>MAQSMYPNEPIVVVGSGCRFPGDANTPSKLWELLQHPRDVQSRIPKERFDVDTFYHPDGKHHGRTNAPYAYVLQDDLGAFDAAFFNIQAGEAESMDPQHRLLLETVYEAVTNAGMRIQDLQGTSTAVYVGVMTHDYETVSTRDLESIPTYSATGVAVSVASNRISYFFDWHGPSMTIDTACSSSLVAVHLAVQQLRTGQSSMAIAAGANLILGPMTFVLESKLSMLSPSGRSRMWDAGADGYARGEAVCSVVLKTLSQALRDGDTIECVIRETGVNQDGRTTGITMPNHSAQEALIKATYAQAGLDITKAEDRCQFFEAHGTGTPAGDPQEAEAIATAFFGHEQVARSDGNERAPLFVGSAKTVVGHTEGTAGLAGLMKASFAVRHGVIPPNLLFDKISPRVAPFYKNLRIPTEATQWPALPPGQPRRASVNSFGFGGTNAHAIIEEYMEPEQNQLRVSNNEDCPPMTGVLSLPLVLSAKSQRSLKIMMEEMLQFLQSHPEIHLHDLTWSLLRKRSVLPFRRAIVGHSHETIRRALEDAIEDGIVSSDFTTEVRGQPSVLGIFTGQGAQWPGMLKNLIEASPYVRNIVRELDDSLQSLPEKYRPSWTLLDQ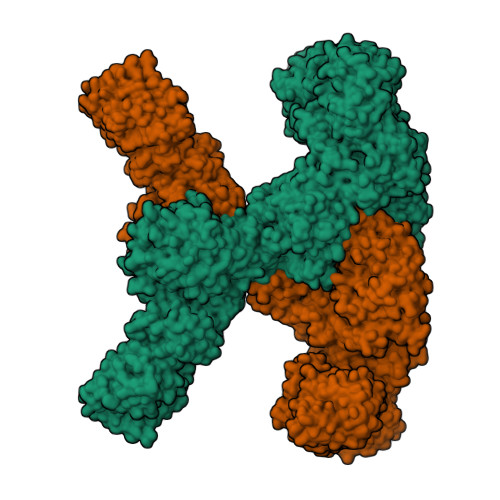FMLEGEASNVQYATFSQPLCCAVQIVLVRLLEAARIRFTAVVGHSSGEIACAFAAGLISASLAIRIAYLRGVVSAGGARGTPGAMLAAGMSFEEAQEICELDAFEGRICVAASNSPDSVTFSGDANAIDHLKGMLEDESTFARLLKVDTAYHSHHMLPCADPYMQALEECGCAVADAGSPAGSVPWYSSVDAENRQMAARDVTAKYWKDNLVSPVLFSHAVQRAVVTHKALDIGIEVGCHPALKSPCVATIKDVLSGVDLAYTGCLERGKNDLDSFSRALAYLWERFGASSFDADEFMRAVAPDRPCMSVSKLLPAYPWDRSRRYWVESRATRHHLRGPKPHLLLGKLSEYSTPLSFQWLNFVRPRDIEWLDGHALQGQTVFPAAGYIVMAMEAALMIAGTHAKQVKLLEILDMSIDKAVIFDDEDSLVELNLTADVSRNAGEAGSMTISFKIDSCLSKEGNLSLSAKGQLALTIEDVNPRTTSASDQHHLPPPEEEHPHMNRVNINAFYHELGLMGYNYSKDFRRLHNMQRADLRASGTLDFIPLMDEGNGCPLLLHPASLDVAFQTVIGAYSSPGDRRLRCLYVPTHVDRITLVPSLCLATAESGCEKVAFNTINTYDKGDYLSGDIVVFDAEQTTLFQVENITFKPFSPPDASTDHAMFARWSWGPLTPDSLLDNPEYWATAQDKEAIPIIERIVYFYIRSFLSQLTLEERQQAAFHLQKQIEWLEQVLASAKEGRHLWYDPGWENDTEAQIEHLCTANSYHPHVRLVQRVGQHLLPTVRSNGNPFDLLDHDGLLTEFYTNTLSFGPALHYARELVAQIAHRYQSMDILEIGAGTGGATKYVLATPQLGFNSYTYTDISTGFFEQAREQFAPFEDRMVFEPLDIRRSPAEQGFEPHAYDLIIASNVLHATPDLEKTMAHARSLLKPGGQMVILEITHKEHTRLGFIFGLFADWWAGVDDGRCTEPFVSFDRWDAILKRVGFSGVDSRTTDRDANLFPTSVFSTHAIDATVEYLDAPLASSGTVKDSYPPLVVVGGQTPQSQRLLNDIKAIMPPRPLQTYKRLVDLLDAEELPMKSTFVMLTELDEELFAGLTEETFEATKLLLTYASNTVWLTENAWVQHPHQASTIGMLRSIRREHPDLGVHVLDVDAVETFDATFLVEQVLRLEEHTDELASSTTWTQEPEVSWCKGRPWIPRLKRDLARNNRMNSSRRPIYEMIDSSRAPVALQTARDSSSYFLESAETWFVPESVQQMETKTIYVHFSCPHALRVQALGFFYLVQGHVQEGNREVPVVALAERNASIVHVRPDYIYTEADNNLSEGGGSLMVTVLAAAVLAETVISTAKCLGVTDSILVLNPPSICGQMLLHAGEEIGLQVHLATTSGNRSSVSAGDAKSWLTLHARDTDWHLRRVLPRGVQALVDLSADQSCEGLTQRMMKVLMPGCAHYRAADLFTDTVSTELHSGSRHQASLPAAYWEHVVSLARQGLPSVSEGWEVMPCTQFAAHADKTRPDLSTVISWPRESDEATLPTRVRSIDAETLFAADKTYLLVGLTGDLGRSLGRWMVQHGACHIVLTSRNPQVNPKWLAHVEELGGRVTVLSMDVTSQNSVEAGLAKLKDLHLPPVGGIAFGPLVLQDVMLNNMELPMMEMVLNPKVEGVRILHEKFSDPTSSNPLDFFVMFSSIVAVMGNPGQANYSAANCYLQALAQQRVASGLAASTIDIGAVYGVGFVTRAELEEDFNAIRFMFDSVEEHELHTLFAEAVVAGRRAVHQQEQQRKFATVLDMADLELTTGIPPLDPALKDRITFFDDPRIGNLKIPEYRGAKAGEGAAGSKGSVKEQLLQATNLDQVRQIVIDGLSAKLQVTLQIPDGESVHPTIPLIDQGVDSLGAVTVGTWFSKQLYLDLPLLKVLGGASITDLANEAAARLPPSSIPLVAATDGGAESTDNTSENEVSGREDTDLSAAATITEPSSADEDDTEPGDEDVPRSHHPLSLGQEYSWRIQQGAEDPTVFNNTIGMFMKGSIDLKRLYKALRAVLRRHEIFRTGFANVDENGMAQLVFGQTKNKVQTIQVSDRAGAEEGYRQLVQTRYNPAAGDTLRLVDFFWGQDDHLLVVAYHRLVGDGSTTENIFVEAGQLYDGTSLSPHVPQFADLAARQRAMLEDGRMEEDLAYWKKMHYRPSSIPVLPLMRPLVGNSSRSDTPNFQHCGPWQQHEAVARLDPMVAFRIKERSRKHKATPMQFYLAAYQVLLARLTDSTDLTVGLADTNRATVDEMAAMGFFANLLPLRFRDFRPHITFGEHLIATRDLVREALQHARVPYGVLLDQLGLEVPVPTSNQPAPLFQAVFDYKQGQAESGTIGGAKITEVIATRERTPYDVVLEMSDDPTKDPLLTAKLQSSRYEAHHPQAFLESYMSLLSMFSMNPALKLAHVHHHHHH[2x]>MTNIVGRIGFLTTGKLGIKLRGVLIDESTTPNTTYLPGIESFFNITANVLTSVSYPETETQNVTATFSIYSVDGSSNPVFPALLSFDAIVPNVASVEFDVLAPTGVVNNQLDTSALRIAKIIANDPALAQKVAGAPYPRGAYSATETYLYGEMVSYFGKNYISKSLSPIINILPTVTDSWYELVITLPESVSVIATGSDTAYGTGWNGSLLVPTQNAVYDKIVTVDAAIATANTNITNLGTAKADLSYVNTQLSADQVVLD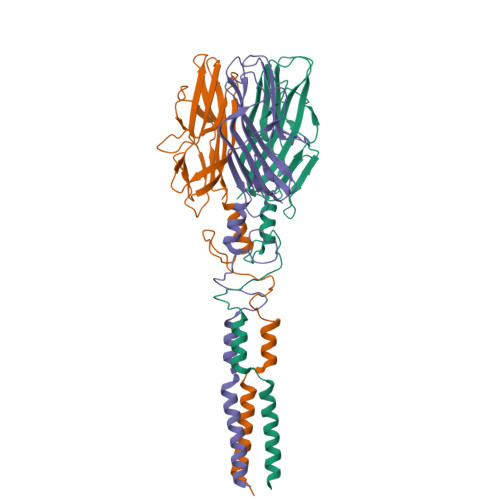ALSSGKADLSYVNTQLNSKANLNGAVLVNATTATPPISDNDTSLATTQHVRSFNHSRLAFNAFRGGQQGVPSLSYVTTTAQFNSSSVRSGWGDNFSSNRWLVGEGGTYLITVTTRFATVGGTPPTYFDALLFVGLSGSGVENFLTRSQSVYPSFGYTLSWVGILTFNTGQNVFLNYQVNAVGGGSYSVVLEDVRFSGIQLG[3x]>[6x]MSRAKAAPVAGPEVAANRAGRQARIVAILSSAQVRSQNELAALLAAEGIEVTQATLSRDLEELGAVKLRGADGGTGIYVVPEDGSPVRGVSGGTDRMARLLGELLVSTDDSGNLAV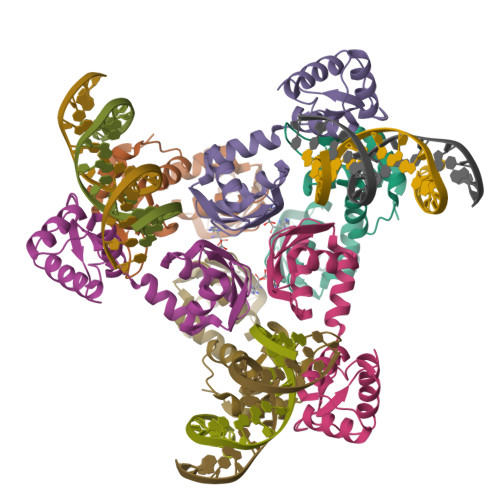LRTPPGAAHYLASAIDRAALPQVVGTIAGDDTILVVAREPTTGAQLAGMFENLR>[4x]GGPIPYPVGNLLHTAPCGFVVTDAVEPDQPIIYVNTVFEMVTGYRAEEVLGRNCRFLQCRGPFAKRRHPLVDSMVVSEIRKCIDEGIEFQ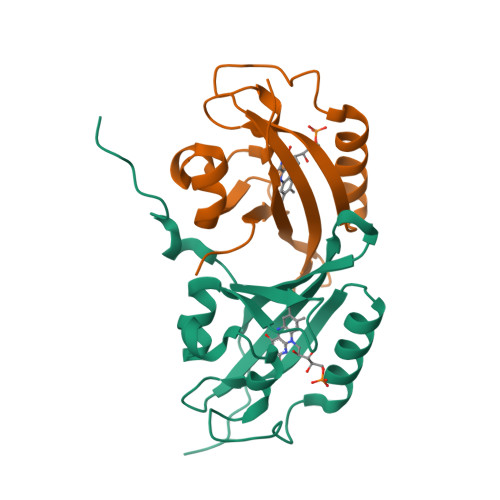GELLNFRKDGSPLMNRLRLTPIYGDDDTITHIIGIQFFIETDIDLGP>HSVAVIGAPFSQGQKRKGVEHGPAAIREAGLMKRLSSLGCHLKDFGDLSFTPVPKDDLYNNLIVNPRSVGLANQELAEVVSRAVSDGYSCVTLGGDHSLAIGTISGHARHCPDLCVVWVDAHADINTPLTTSSGNLHGQPVSFLLRELQDKVPQLPGFSWIKPCISSASI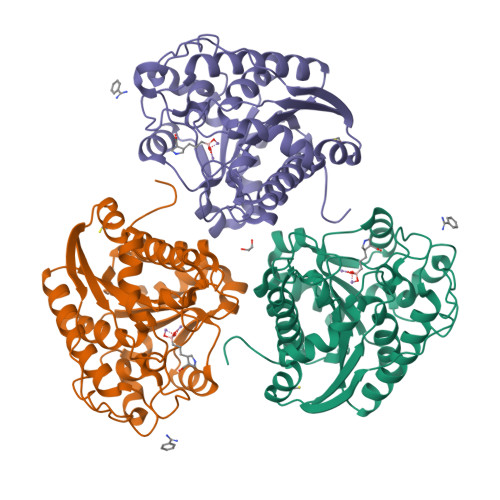VYIGLRDVDPPEHFILKNYDIQYFSMRDIDRLGIQKVMERTFDLLIGKRQRPIHLSFDIDAFDPTLAPATGTPVVGGLTYREGMYIAEEIHNTGLLSALDLVEVNPQLATSEEEAKTTANLAVDVIASSFGQTREG[3x]> SAAANDVNYSFDEAVSMQQGKGIVQTKEEDGKFVEANNNEIAKAMTISHKDNDMKYMDITEKVPMSESEVNQLLKGKGILENRGKVFLEAQEKYEVNVIYLVSHALVATGNGKSELAKGIKDGKKRYYNFFGIGAF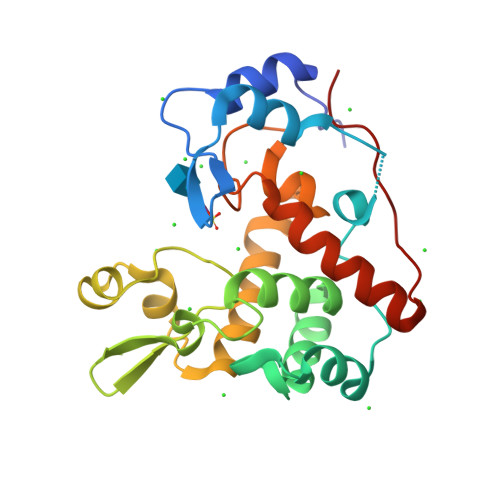DSSAVRSGKSYAEKEQWTSPDKAIIGGAKFIRNEYFENNQLNLYQMRWNPENPAQHQYASDIRWADKIAKLMDKSYKQFGIKKDDIRQTYYK> MTAIVEAPQPGAEAIASPQAAVVAIMAADVQIAVVLDAHAPISVMIDPLLKVVNTRLRELGVAPLEAKGRGRWMLCLVDGTPLRPNLSLTEQEVYDGDRLWLKFLEDTEHRSEVIEHISTAVATNLSKRFAPIDPVVAVQVGATMVAVGVLLGSALLGWWRWQHESWLPAPFAAVIAVLVLTVATMILARSKTVPDRRVGDILLLSGLVPLAVAIAATAPGPVGAPHAVLGFGVFGVAAMLVMRFTGRRLGVYTALVTLCAAATAAGLARMVLLTSAVTLLTCVLLACVLMYHGAPALSRWLSGIRLPVFPSATSRWVFEARPDLPTTVVVSGGGQPTLEGPASVRDVLLRAERARSFLTGLLVGLGVLTVVCLAGLCDPHAGRRW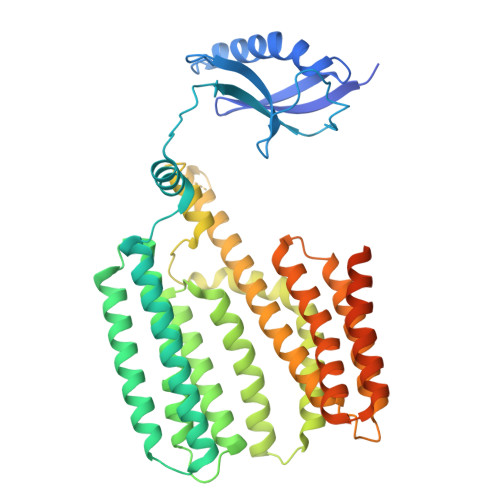LPLLLAAFTFGFLILRGRSYVDRWQAITLAATAVLIIAAVAVRYVLVSGSPAVLSAGVAVLVLLPAAGLTAAAVVPNTIYSPLFRKIVEWIEYLCLMPIFPLALWLMNVYEAIRYR> SNAQSEQSTHIEGVAEKPVEFVKLGTGVWMHTGYKVVPPWGNIRTNGLIIERGDYSVLVDTAWNDAQTAEIVAWAKDTLQKPIRASIHTHAHSDKMGGMDALHMLGVETFATDLTNRLAIERGLMPAKNVLNISEIGSQIEWEGLTILYPGGGHSEDNIVVNEGVNNILFGGCMIRPGMTTSLG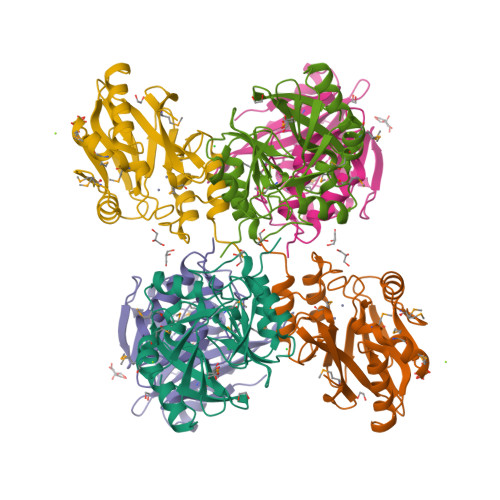NIDDANLGYWSKAVENAANAFPDSQIVIPSHGKPAGREILKNTAYITRPKL>QDPLSCYDNFGNRDVAACARFIDDFCDTLTPNIYRPRDNGQRCYVVNGHKCDFTVFNTNNGGSPIRASTPNCKTV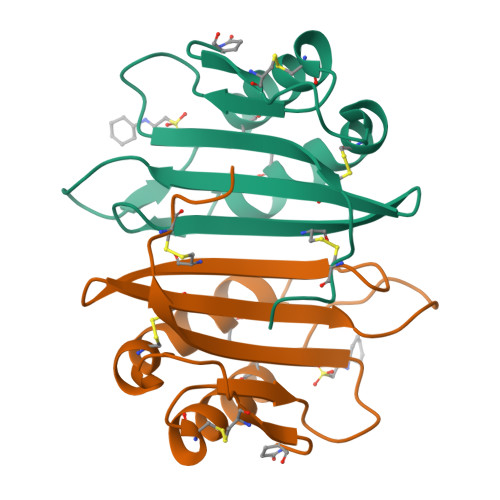LRAAANRCPTGGRGKINPSAPFLFAIDPNDGDCSTDF[4x]>MGKLLLILGSAIALPSFAAAGGDLDISDTVGVSFWLVTAGMLAATVFFFVERDQVSAKWKTSLTVSGLITGIAFWHYLYMRGVWIDTGDTPTVFRYINWLLTVPLLVVEFYLILAACTSVAASLFKKLLAGSLVMLGAGFAGEAGLAPVLPAFIIGMAGWLYMIYELYMGEGKAAVSTASPAVNSAYNAMMMIIVVGWAIYPAGYAAGYLMGGEGVYASNLNLIYNLADFVNKILFGLIIWNVAVK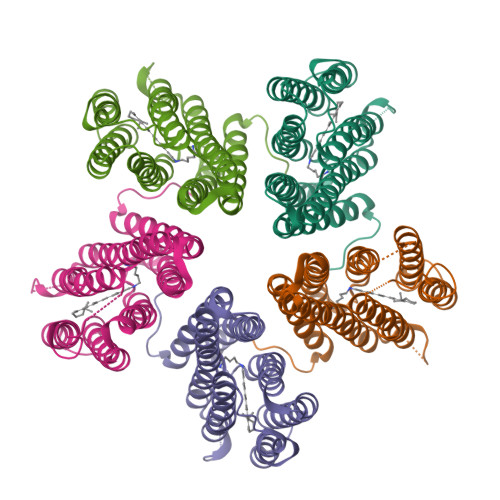ESSNAKLLEHHHHHH[5x]> GSLKIAPANADFAFRFYYLIASETPGKNIFFSPLSISAAYAMLSLGACSHSRSQILEGLGFNLTELSESDVHRGFQHLLHTLNLPGHGLETRVGSALFLSHNLKFLAKFLNDTMAVYEAKLFHTNFYDTVGTIQLINDHVKKETRGKIVDLVSELKKDVLMVLVNYIYFKALWEKPFISSRTTPKDFYVDENTTVRVPMMLQDQEHHWYLHDRYLPCSVLRMDYKGDATVFFILPNQGKMREIEEVLTPEMLMRWNNLLRKRNFYKKLELHLPKFSISGSYVLDQILPRLGFTDLFSKWADLSGITKQQKLEASKSFHKATLDVDEAGTEAAAATS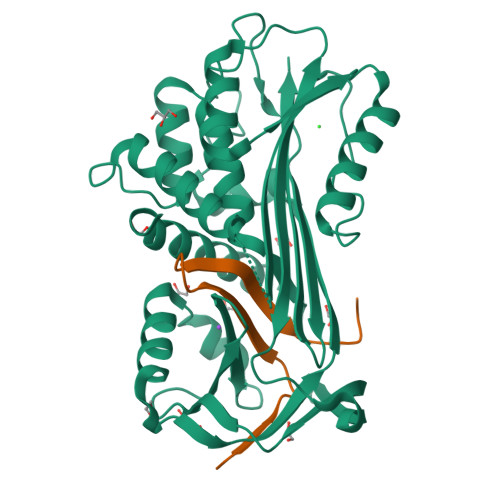FAIKF;> FSAQTNRHILRFNRPFLVVIFSTSTQSVLFLGKVVDPTKP>[4x]MTTAAIRGLQGEAPTKNKELLNWIADAVELFQPEAVVFVDGSQAEWDRMAEDLVEAGTLIKLNEEKRPNSYLARSNPSDVARVESRTFICSEKEEDAGPTNNWAPPQAMKDEMSKHYAGSMKGRTMYVVPFCMGPISDPDPKLGVQLTDSEYVVMSMRIMTRMGIEALDKIGANGSFVRCLHSVGAPLEPGQEDVAWPCNDTKYITQFPETKEIWSYGSGYGGNAILAKKCYALRIASVMAREEGWMAEHMLILKLINPEGKAYHIAAAFPSACGKTNLAMITPTIPGWTAQVVGDDIAWLKLREDGLYAVNPENGFFGVAPGTNYASNPIAMKTMEPGNTLFTNVALTDDGDIWWEGMDGDAPAHLIDWMGNDWTPESDENAAHPNSRYCVAIDQSPAAAPEFNDWEGVKIDAILFGGRRADTVPLVTQTYDWEHG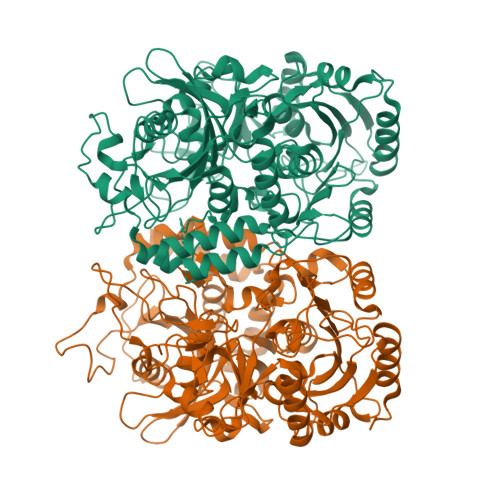TMVGALLASGQTAASAEAKVGTLRHDPMAMLPFIGYNAGEYLQNWIDMGNKGGDKMPSIFLVNWFRRGEDGRFLWPGFGDNSRVLKWVIDRIEGHVGADETVVGHTAKAEDLDLDGLDTPIEDVKEALTAPAEQWANDVEDNAEYLTFLGPRVPAEVHSQFDALKARISAAHA>[2x]MTVLATSRLHI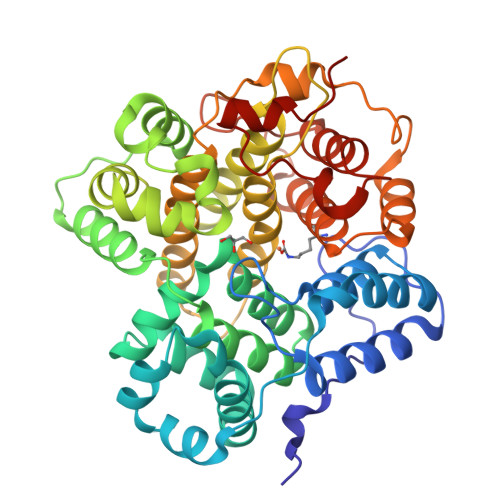EGDFRGYGSLDKSPPGALETLNRLMQNNHDEFDMFWRPDAGHNHTAFSLLSVYALGGSSADLERAYRDDDPHQVPIGAVDHSVVASLKDPRIFIHRMQRLDQYSNYLRFFEERIEARGWKAVVVEYLFSRSDAAEAMLGQLFEGAYHPLIQLGFGIEFELPGLVAEGLAHCAAHDAANIIPFFQKAEKLAKSGSVAPAPLVELYKEVRDTEKIRLAAKMTQGPVRVRDGVMGEAQDDIAAVAAKFQVGPDGLKQAIIETTSCAAYSCGGAQRPGKVAKVDFFFMHMVTSSIFLSILARQDWLETEDKIRLVEWKGRLDLVWYAASSAPALDRKWLEQYQPTLSAGMDWRALYRAVTVEPDDGHLAKIVRSLKWAEEEAKGVETSETIPVAGSGWFKLAQMAYDSTAHLPIPAKWIMGAGYDFLWTRVDSLPAA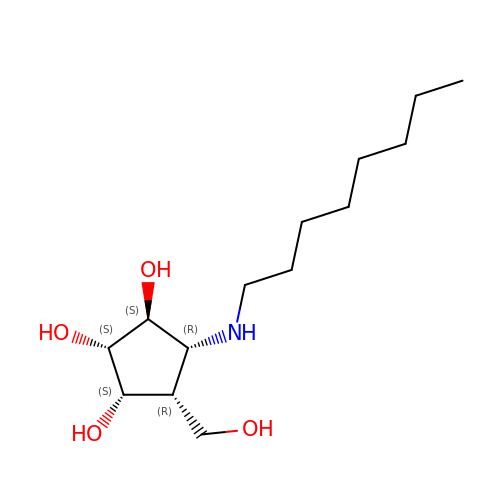(1~{S},2~{S},3~{S},4~{R},5~{R})-4-(hydroxymethyl)-5-(octylamino)cyclopentane-1,2,3-triol | C14 H29 N O4 | UZTOTQLQFAGSAI-NDKCEZKHSA-N> MKALGRGPITRLANTAAPGGFAAPGAVYNRDDWNAGRDVSAEERQCGILTRLCTLAATAPREAASPACGLAPLEAVIR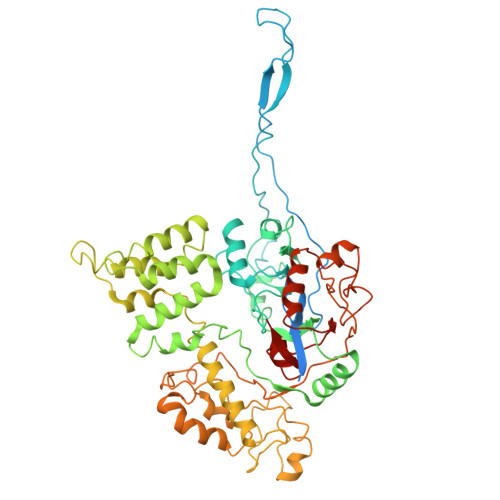VQSTDAHVTEVDANGGGAFLEKAPKGRWRKISRSKTLLVEDTATPFSNSDKSFSPRVQSYGEYVRRIGKLPEGRPLLRFAMFRDGYSLDSVCHRLRYEIGVPHDGVYLHEPPGGSFAAVTQFGVAVGVTREQLPHASRHYNVHALIFDDRGYHALDELPRLSVAPQAYLHRILLRCVSGDEAAVAQRLRHLSSNGFINYFGLESFGIGSNTLFDMAAFAFRREPHRSVGAYLQTLAECSPLHHQPYLSYANAEESTVAGAVAEWLRVCERAKLPRETRELLRKLHCYHLSQCHPSDATTISMEDVWKACPIMHRAEQSAAAFVWNAMASQRLLSFGSRPVKGDLVCRIGNRGAIEIAEVASDTDASHYTIDDVVLPIPCGGTPAAELRYPTHSVNEAFFTQFAKKHSLSFLFNSGVDPTPRAAATLGPYRRLVSRPRNLQAAVLQDPSSCAALKSDLFLLQEHQPTEGWSLDYRQRVREPSNFNVSERFRERMSCIRKRRAGEHSVALAFVLPAGSSPWVALREAFHMHYGTFHDFYGVS>[2x]LAMTMEHKDRPLVRVILTNTGSHPVKQRSVYITALLDSGADITIISEEDWPTDWPVMEAANPQIHGIGGGIPMRKSRDMIELGVINRDGSL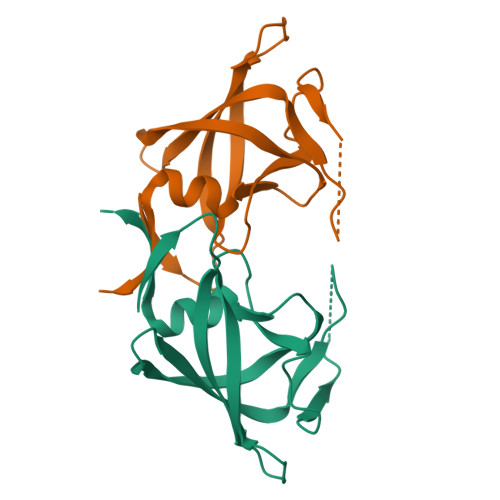ERPLLLFPAVAMVRGSILGRDCLQGLGLRLTNL> TV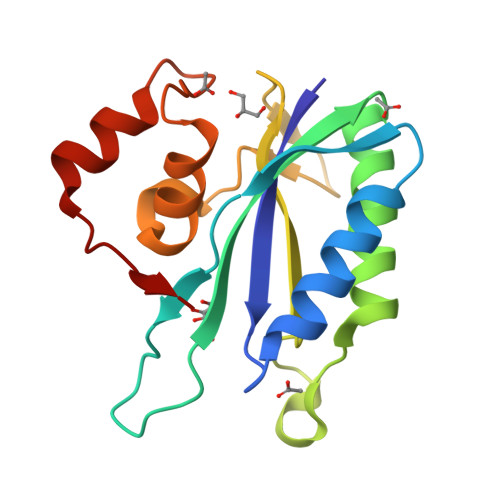AYIAIGSNLASPLEQVNAALKALGDIPESHILTVSSFYRTPPLGPQDQPDYLAAAVALETSLAPEELLNHTQRIELQQGRVRKAERWGPRTLDLDIMLFGNEVINTERLTVPHYDMKNRGFMLWPLFEIAPELVFPDGEMLRQILHTRAFDKLNKW> AASAQDAPEAETQAQETQGQA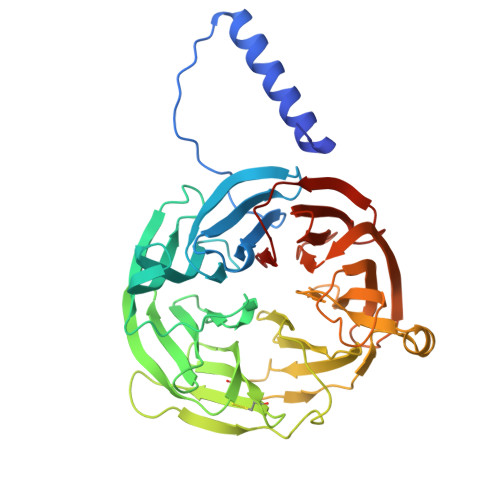AARAAAADLAAGQDDEPRILEAPAPDARRVYVNDPAHAAAVTQQFVIDGEAGRVIGMIDGGFLPNPVVADDGSFIAHASTVFSRIARGERTDYVEVFDPVTLLPTADIELPDAPRFLVGTYPWMTSLTPDGKTLLFYQFSPAPAVGVVDLEGKAFKRMLDVPDCYHIFPTAPDTFFMHCRDGSLAKVAFGTEGTPEITHTEVFHPEDEFLINHPAYSQKAGRLVWPTYTGKIHQIDLSSGDAKFLPAVEALTEAERADGWRPGGWQQVAYHRALDRIYLLVDQRDEWRHKTASRFVVVLDAKTGERLAKFEMGHEIDSINVSQDEKPLLYALSTGDKTLYIHDAESGEELRSVNQLGHGPQVITTADMG> GGAGAGUAGAUGAUUCGCGUUAAGCGUGUGUGAAUGGGAUGUCGUCACACAACGAAGCGAGAGCGCG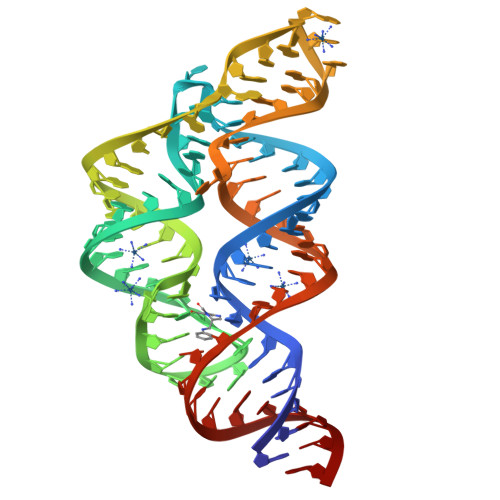GUGAAUCAUUGCAUCCGCUCCA> GSGSWQTYVDEHLMCDIEGTGQHLASAAIFGTDGNVWAKSSSFPEFKP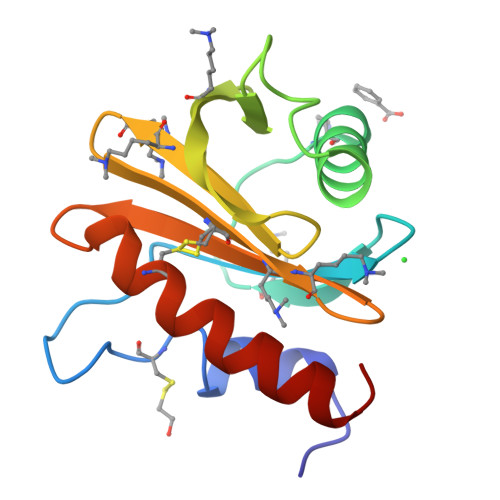DEINAIIKEFSEPGALAPTGLFLAGAKYMVIQGEPGAVIRGKKGAGGICIKKTGQAMVFGIYEEPVNPGQCNMVVERLGDYLVDQGM> VLSSQNKKAIEELGNLIKANAEAWGADA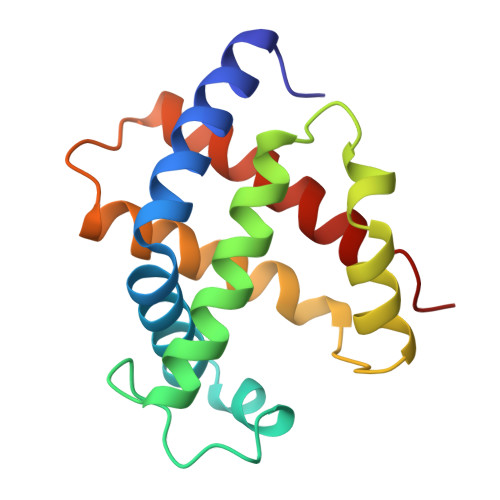LARLFELHPQTKTYFSKFSGFEACNEQVKKHGKRVMNALADATHHLDNLHLHLEDLARKHGENLLVDPHNFHLFADCIVVTLAVNLQAFTPVTHCAVDKFLELVAYELSSCYR> SAFSAF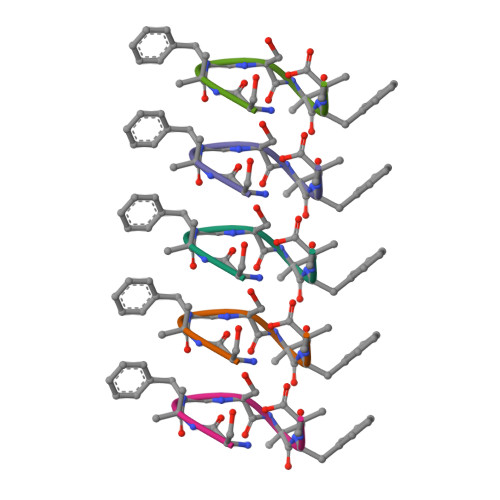A> 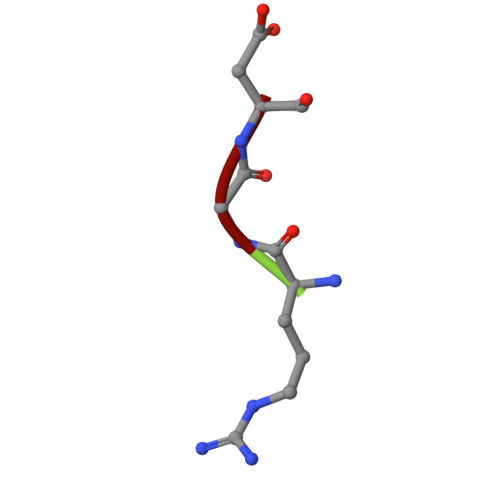RGD3-(benzyloxy)-5-methyl-N-(4-methyl-1,3-thiazol-2-yl)pyridin-2-amine | C17 H17 N3 O S | 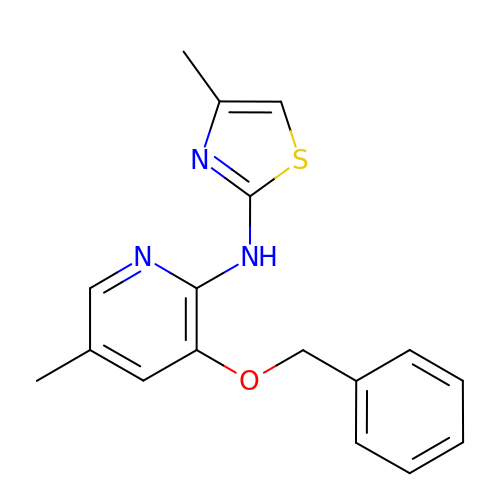QFOFZZJJRFMLKB-UHFFFAOYSA-N> MSNFIFGRYLPLDSVVHRLDPRAKLMLSFCYIIVVFLANNIWSYAILIAFTVGAILSSKISLGFFLKGIRPLLWLIVFTVVLQLLFSPAGGHTYFHWAFINVTQDGLINAGYIFVRFLLIIMMSTLLTLSTQPLDIATGLASLMKPLRWVKVPVDTLAMMLSIALRFVPTLMDEATKIMNAQRARGVDFGEGGLFKQAKSLIPLMVPLFMSAFNRAEDLSTAMEAR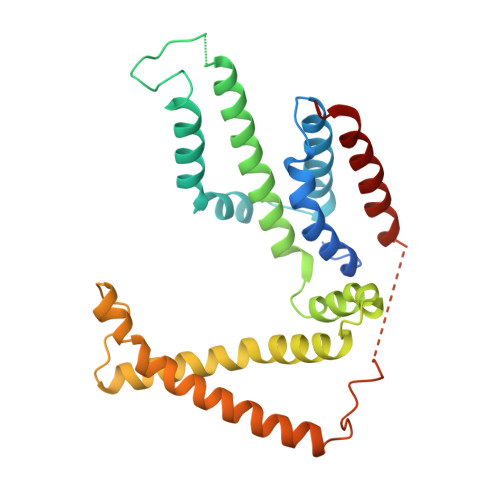GYQDSEHRSQYRILTWQRRDTVTWLLFLLGFVAILIFRHW> MTQAKAKHADVPVNLYRPNAPFIGKVISNEPLVKEGGIGIVQHIKFDLTGGNLKYIEGQSIGIIPPGVDKNGKPEKLRLYSIASTRHGDDVDDKTISLCVRQLEYKHPESGETVYGVCSTYLTHIEPGSEVKITGPVGKEMLLPDDPEANVIMLATGTGIAPMRTYLWRMFKDAERAANPEYQFKGFSWLVFGVPTTPNILYKEELEEIQQKYPDNFRLTYAISREQKNPQGGRMYIQDRVAEHADQLWQLIKNEKTHTYICGLRGMEEGIDAALSAAAAKEGVTWSDYQ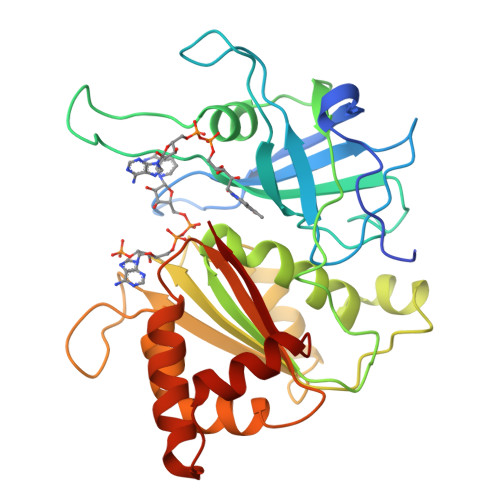KDLKKAGRWHVETY>MKSTSDLFNEIIPLGRLIHMVNQKKDR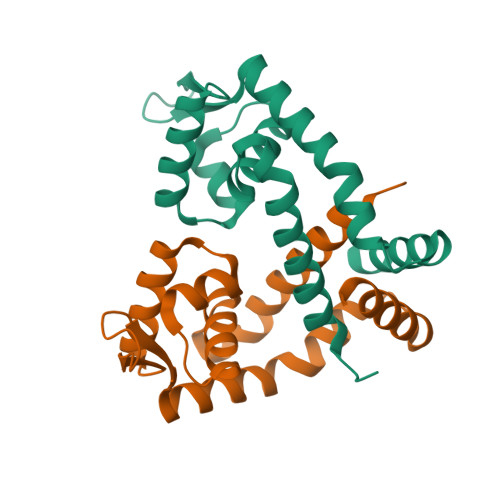LLNEYLSPLDITAAQFKVLCSIRCAACITPVELKKVLSVDLGALTRMLDRLVSKGWVERLPNPNDKRGVLVKLTTGGAAICEQCHQLVGQDLHQELTKNLTADEVATLEYLLKKVLP[2x]~{N}-[2-(2,4-dimethylphenyl)-4,6-dihydrothieno[3,4-c]pyrazol-3-yl]-3,4-dimethyl-benzamide | C22 H23 N3 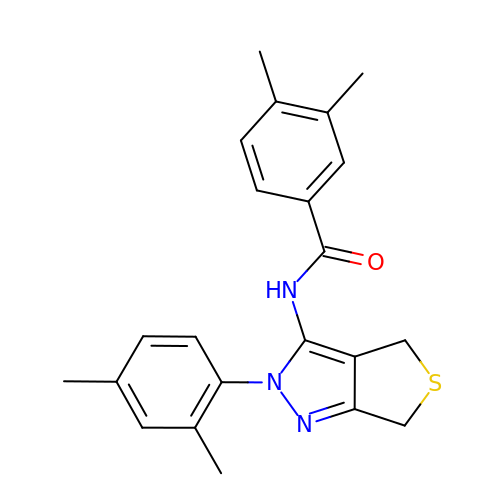O S | FJKKXWLUKJOWNU-UHFFFAOYSA-N> MSADAQSFLNRVCGVSAARLTPCGTGTSTDVVYRAFDIYNDKVAGFAKFLKTNCCRFQEKDEDDNLIDSYFVVKRHTFSNYQHEETIYNLLKDCPAVAKHDFFKFRIDGDMVPHISRQRLTKYTMADLVYALRHFDEGNCDTLKEILVTYNCCDDDYFNKKDWYDFVENPDILRVYANLGERVRQALLKTVQFCDAMRNAGIVGVLTLDNQDLNGNWYDFGDFIQTTPGSGVPVVDSYYSLLMPILTLTRALTAESHVDTDLTKPYIKWDLLKYDFTEERLKLFDRYFKYWDQTYHPNCVNCLDDRCILHCANFNVLFSTVFPPTSFGPLVRKIFVDGVPFVVSTGYHFRELGVVHNQDVNLHSSRLSFKELLVYAADPAMHAASGNLLLDKRTTCFSVAALTNNVAFQTVKPGNFNKDFYDFAVSKGFFKEGSSVELKHFFFAQDGNAAISDYDYYRYNLPTMCDIRQLLFVVEVVDKYFDCYDGGCINANQVIVNNLDKSAGFPFNKWGKARLYYDSMSYEDQDALFAYTKRNVIPTITQMNLKYAISAKNRARTVAGVSICSTMTNRQFHQKLLKSIAATRGATVVIGTSKFYGGWHNMLKTVYSDVENPHLMGWDYPKCDRAMPNMLRIMASLVLARKHTTCCSLSHRFYRLANECAQVLSEMVMCGGSLYVKPGGTSSGDATTAYANSVFNICQAVTANVNALLSTDGNKIADKYVRNLQHRLYECLYRNRDVDTDFVNEFYAYLRKHFSMMILSDDAVVCFNSTYASQGLVASIKNFKSVLYYQNNVFMSEAKCWTETDLTKGPHEFCSQHTMLVKQGDDYVYLPYPDPSRILGAGCFVDDIVKTDGTLMIERFVSLAIDAYPLTKHPNQEYADVFHLYLQYIRKLHDELTGHMLDMYSVMLTNDNTSRYWEPEFYEAMYTPHTVLQGGSENLYFQGHHHHHHHH;> MAIASEFSSLPSYAAFATAQEAYEQAVANGDSEVVLKKLKKSLNVAKSEFDRDAAMQRKLEKMADQAMTQMYKQARSEDKRAKVTSAMQTMLFTMLRKLDNDALNNIINNARDGCVPLNIIPLTTAAKLMVVIPDYNTYKNTCDGTTFTYASALWEIQQVVDADSKIVQLSEISMDNSPNLAWPLIVTALRANSAVK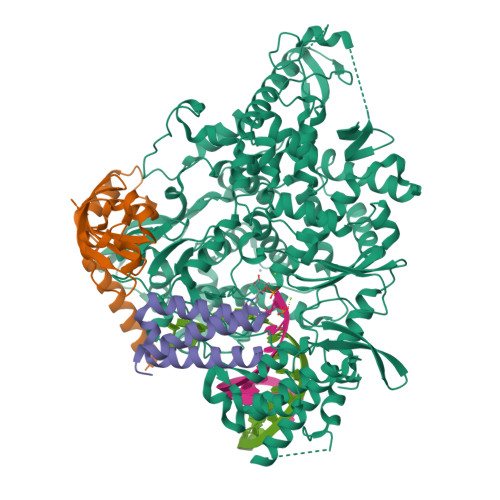LQHHHHHHHH;> MSKMSDVKCTSVVLLSVLQQLRVESSSKLWAQCVQLHNDILLAKDTTEAFEKMVSLLSVLLSMQGAVDINKLCEEMLDNRATLQHHHHHHHH>MGSSHHHHHHSSGLVPRGSPTYVGKEAPFFKAEAVFGDNSFGEVNLTQFIGKKYVLLYFYPLDFTFVCPSEIIALDKALDAFHERNVELLGCSVDSKYTHLAWKKTPLAKGGIGNIKHTLLSDITKSISKDYNVLFDDSVSLRAFVLIDMNGIVQHLLVNNLAIGRSVDEILRIIDAIQHHEKYGDVCPANWQKGKVSMKPSEEGVAQYLS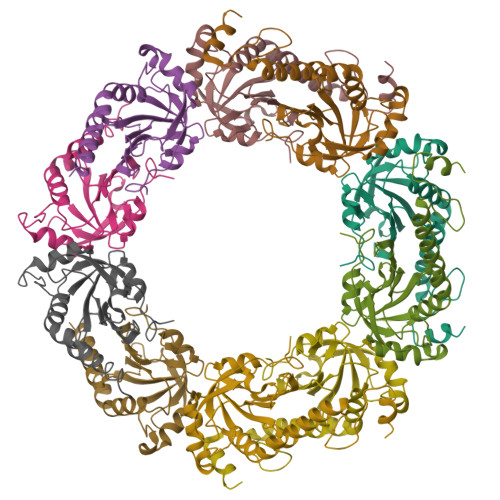TL[5x]> MELKHSISDYTEAEFLEFVKKICRAEGATEEDDNKLVREFERLTEHPDGSDLIYYPRDDREDSPEGIVKEIKEWRAANGKSGFKQGLEHHHHH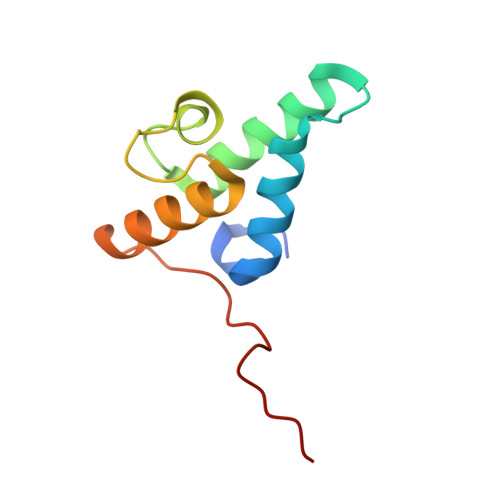H> MMFGKKKNNGGSSTARYSAGNKYNTLSNNYALSAQQLLNASKIDDIDSMMGFERYVPPQYNGRFDAKDIDQIPGRVGWLTNMHATLVSQETLSSGSNGGGNSNDGERVTTNQGISGVDFYFLDEEGGSFKSTVVYDPYFFIACNDESRVNDVEELVKKYLESCLKSLQIIRKEDLTMDNHLLGLQKTLIKLSFVNSNQLFEARKLLRPILQDNANNNVQRNIYNVAANGSEKVDAKHLIEDIREYDVPYHVRVSIDKDIRVGKWYKVTQQGFIEDTRKIAFADPVVMAFAIATTKPPLKFPDSAVDQIMMISYMIDGEGFLITNREIISEDIEDFEYTPKPEYPGFFTIFNENDEVALLQRFFEHIRDVRPTVISTFNGDFFDWPFIHNRSKIHGLDMFDEIGFAPDAEGEYKSSYCSHMDCFRWVKRDSYLPQGSQGLKAVTQSKLGYNPIELDPELMTPYAFEKPQHLSEYSVSDAVATYYLYMKYVHPFIFSLCTIIPLNPDETLRKGTGTLCEMLLMVQAYQHNILLPNKHTDPIERFYDGHLLESETYVGGHVESLEAGVFRSDLKNEFKIDPSAIDELLQELPEALKFSVEVENKSSVDKVTNFEEIKNQITQKLLELKENNIRNELPLIYHVDVASMYPNIMTTNRLQPDSIKAERDCASCDFNRPGKTCARKLKWAWRGEFFPSKMDEYNMIKRALQNETFPNKNKFSKKKVLTFDELSYADQVIHIKKRLTEYSRKVYHRVKVSEIVEREAIVCQRENPFYVDTVKSFRDRRYEFKGLAKTWKGNLSKIDPSDKHARDEAKKMIVLYDSLQLAHKVILNSFYGYVMRKGSRWYSMEMAGITCLTGATIIQMARALVERVGRPLELDTDGIWCILPKSFPETYFFTLENGKKLY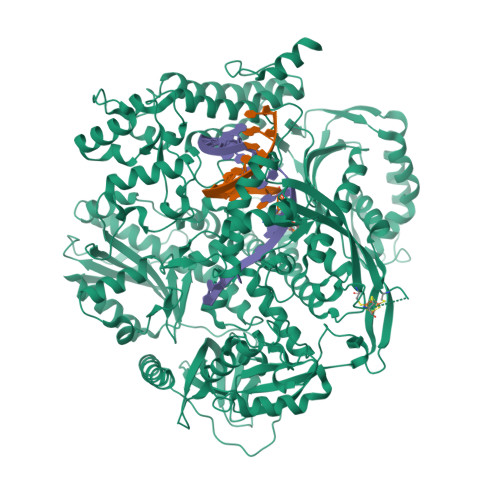LSYPCSMLNYRVHQKFTNHQYQELKDPLNYIYETHSENTIFFEVDGPYKAMILPSSKEEGKGIKKRYAVFNEDGSLAELKGFELKRRGELQLIKNFQSDIFKVFLEGDTLEGCYSAVASVCNRWLDVLDSHGLMLEDEDLVSLICENRSMSKTLKEYEGQKSTSITTARRLGDFLGEDMVKDKGLQCKYIISSKPFNAPVTERAIPVAIFSADIPIKRSFLRRWTLDPSLEDLDIRTIIDWGYYRERLGSAIQKIITIPAALQGVSNPVPRVEHPDWLKRKIATK> GPMGSMNNNEPDTLPDPAIGYIFQNDIVALKQAFSLPDI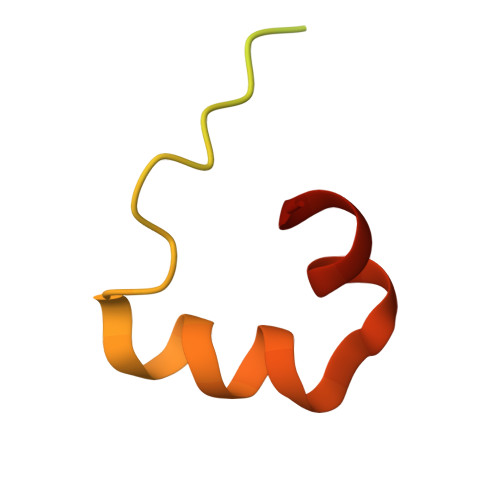DYADISQREQLAAALKRWPLLAEFAQQK> CLAVPGKVIEVNGPVAVVDFGGVKREVRLDLMPDTKPGDWVIVHTGFAIEKLDEKKAMEILEAWAEVEKAMEGF;> MEEPFEAYRSREVAMKLVEKIREEAKTLDGEIRIMHVCGTHEDTVTRHGIRSLLPENVKVVSGPGCPVCITPVEDIVAMQLIMRKAREEGEEIILTTFGDMYKIPTPMGSFADLKSEGFDVRIVYGIFDTYRIAKENPDKTVVHFSPGFETTTAPAAGMLNVAAQEELENFKIYSVHRLTPPAVEVLLKQGTVFQGLIAPGHVSTIIGVKGWEYLTEKYGIPQVVAGFEPNDVLMAILMLIRMYKEGEARIINEYERAVKYEGNVVAQKMIDKFFEVVDAKWRALGVFPKSGLELRKEWKDFEIRSFYKVEVPKNLPDLEKGCRCGAVLRGLALPTDCPLFGKTCTPRHPVGPCMVSYEGTCQIFYKYGV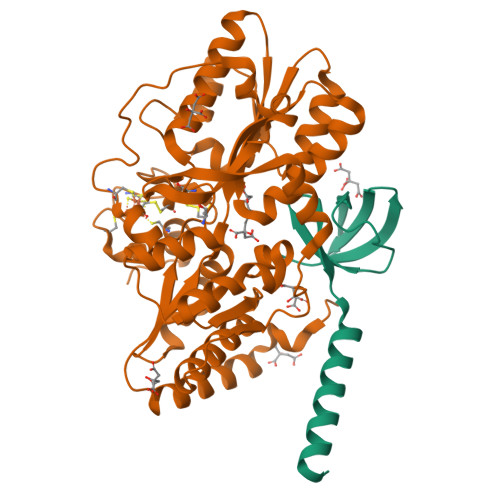LF>[2x]MTKYFDYAASTPVAKGVLESMKPWQSDSFANPSAAHIEAEKALNAIKQAREIIADTLGAMPSEIVFTCGASESNNLAIKGLAFKRLEEKGHLITSSIEHKCVLN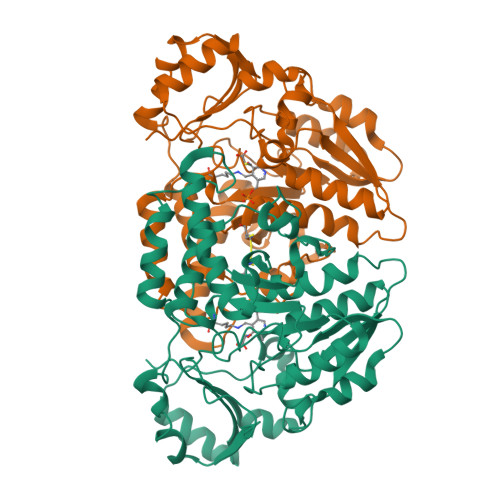TCGFLESIGFDVTYLTPKASGLISAQQVEEAIRPNTFLITIHHVNNELGTVQPIEDIGNVAFEHDIPFHTDAAQSFCKLDIDVDDMNIDMLSLSGHKVYGPKGIGALYVRDARNSELVPLIHGGGQELGLRGGTSPTPLIVGLGVAVEHFPSEASAQQTEFEKIINEYSFSRNSGDNALSTTWNVTFENDDEVKRFTSERNWLISQGSASNAMSNTPSHVLTAIGLSEAEARRTYRISLPPYKV>MKTSKWIDISQPLNNDIATWPGDTPFSYEVLWSKEESGSVNVGKLTMSIHTGTHIDAPFHFDNDGKKVLDLDIQVYVGPTRIIDVSNLESIGKKELEKFHLEGVERLLLRTSSHGKANEFPDIIPHLRADIAPFLSEKGIRLIGVDVPSVDPLDDKELAAHHQLFKHSIHILENVVLDHVADGDYELIALPLALSDADGSPVRAVIRPI[4x]

The proteins involved in tryptophan catabolism are in general highly conserved across species, but with the notable exception of the second enzyme in the pathway: kynurenine formamidase. This enzyme catalyses the conversion of N-formyl-L-kynurenine (NFK) into formate and L-kynurenine. Our attention was drawn to the prokaryotic KFase KynB (EC 3.5.1.9). The KynB subunit, approximate mass 23 kDa, comprises just over 200 residues with about 50% in 12 β-strands and 15% in four α-helices.

Highly ordered structures of BaKynB and a complex with 2-aminoacetophenone at resolutions of 1.9 and 2.3 Å resulted and confirmed the binuclear Zn2+ environment. We also investigated 2-aminoacetophenone given chemical similarities to part of L-kynurenine. This ligand provides the aromatic component of substrate and product and primarily lacks only the 2-amino-4-oxobutanoic acid moiety. Formate did not elicit any spectroscopic change but L-kynurenine and 2-aminoacetophenone gave comparable Kd values of approximately 60 and 50 μM, respectively. However, the characterization of a BaKynB–2-aminoacetophenone complex structure at 2.25 Å resolution provides a suitable template to inform on aspects of molecular recognition in the active site. Key to ligand, and by implication substrate, binding is the interaction with Trp20. The 2-amino group forms a hydrogen bond to the Zn2+ bridging water or hydroxide. In this respect, the complex derived may closely mimic the configuration at the completion of the catalytic reaction and immediately prior to the replacement of product by the incoming substrate for another round of catalysis. An intramolecular hydrogen bond between the amine and carbonyl groups of 2-aminoacetophenone appeared to be significant. Therefore, such an intramolecular hydrogen bond probably defines or constrains the substrate conformation, and orients the scissile bond such that the formyl moiety would be directed over between His60 and Ser149.To gain insight into the evolution and designability of ligand binding and specificity, we analyzed the homologous PBPs, PotF and PotD, which are Escherichia coli putrescine (PUT)-binding protein and spermidine (SPD)-binding protein, respectively. They constitute the first elements of two separate multicomponent uptake systems (PotFGHI and PotABCD) to transport the cationic polyamines PUT and SPD across the cellular membrane. Still, the protein-binding modes differ: PotF shows affinity for PUT and SPD, whereas PotD exclusively binds SPD. Prior to this work, we grafted the seven differences in amino acids from PotD binding pocket onto PotF; this resulted in PotF_SPD, which will be referred to as PotF/D throughout this work to keep naming for mutants more concise.

Hence, the focus shifted toward D247S, the wildtype Asp bears one of two major carboxyl groups important in primary amine coordination upon ligand binding and recognition in PotF. We introduced the S247D exchange into PotF/D and into our high-affinity constructs E39D–Y87S–F88Y and E39D–F88A/L. PotF/D–S247D showed an improved SPD affinity in the regime of the first-round salt bridge construct (KD(SPD) ≈ 9.4 μM; Table 2). Nonetheless, all constructs regained PUT affinity in the medium to low micromolar range. This was expected as we reintroduced the wildtype-like proximal primary amine–binding site in these variants. All structures but PotF/D–S247D adopt a fully closed wildtype conformation. All in all, we determined salt bridges and the key carboxyl-harboring proximal residue D247 as the basic prerequisites for a complete closure of PotF constructs. Fixing each component by itself was not sufficient. Only the combination of both allows full closure, deeming it an intricately regulated process.

> AEQKTLHIYNWTEYIAPDTVANFEKETGIKVVYDVFDSNEVLEGKLMAGSTGFDLVVPSAYFLERQLTAGVFQPLDKSKLPEWKNLDPELLKLVAKHDPDNKFAMPYMWATTGIGYNVDKVKAVLGENAPVDSWDLILKPENLEKLKSCGVSFLDDPEEVFATVLNYLGKDPNSTKADDYTGPATDLLLKLRPNIRYFHSSQYINDLANGDICVAIGWAGDVWQASNRAKEAKNGVNVSFSIPKEGAMAWFDVFAMPADAKNKDEAYQFLNYLLRPDVVAHISDHVFYANANKAATPLVSAEVRENPGIYPPADVRAKLFTQKVQDPKIDRVRTRAWTKVKSGKLEHHHHHH> IVGGYTCGANTVPYQVSLNSGYHFCGGSLINSQWVVSAAHCYKSGIQVRLGEDNINVVEGNEQFISASK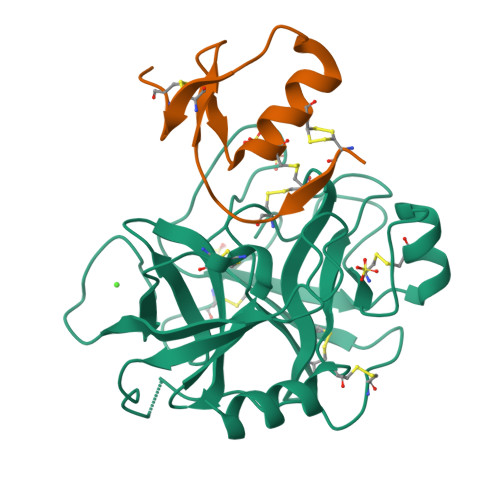SIVHPSYNSNTLNNDIMLIKLKSAASLNSRVASISLPTSCASAGTQCLISGWGNTKSSGTSYPDVLKCLKAPILSDSSCKSAYPGQITSNMFCAGYLEGGKDSCQGDSGGPVVCSGKLQGIVSWGSGCAQKNKPGVYTKVCNYVSWIKQTIASN;> LEENDCACPRVLHRVCGSDGNTYSNPCTLDCAKHEGKPDLVQVHEGPCDPNDHDF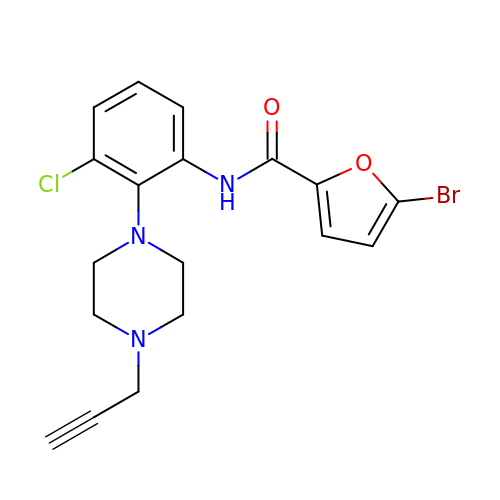5-bromo-N-(3-chloro-2-(4-(prop-2-ynyl)piperazin-1-yl)phenyl)furan-2-carboxamide | C18 H17 Br Cl N3 O2 | MEFJFXHHHNDHEN-UHFFFAOYSA-N> MQGSRKPNIIFIMADDLGWGELGSYGNTFNETPNLDRLSAQGMRFTQAYAAAPVASPTRASIMTGQYPARVGITDFLPEDEKTDRWLDPTKYVTLNEALSASGYHTGIVGKWHLDTDFKLNKGGPKAHGFNEVIGTESEYIADGDYFFPYSKIASFDKGTANEYLTDRQCAEANAFITRNREKPFFLYLSLYSVHTRLEAPVQLVEKYKQKFDQKYGTGKAEQFFGANNVRHESAQRDNPWLAAMLESIDTGVGGI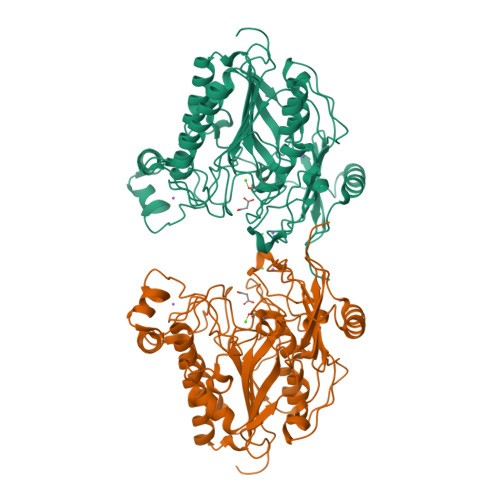MKTLRETGLAENTIIVFFSDNGGAGKAGNNAHLRAGKTWLYEGGIREPLIVSWPGKIKGNTVNDNPVTSLDFYPTFLAAAGGKPTGGRLDGHNLMPLLRGGRASGRPLFWHYPSETGKWVNRMSSAVREGNYKLLEFYNNPRLELYDLQNDPSESHNLATDRPAETARLKKLLEDWKKEVNAEAPHLARKEKKKPGSHHHHHH N-(6-chloro-3,3-dimethyl-3,4-dihydroisoquinolin-1-yl)-3-[4-(1H-pyrazol-4-yl)thiophen-3-yl]-L-alanine | C21 H21 Cl N4 O2 S | 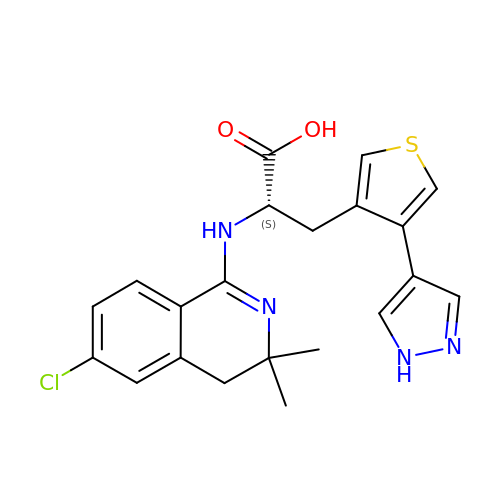ASNJXTHXWLJRAC-SFHVURJKSA-N N-({4-[(1S)-4-(2,4-diamino-6-oxo-1,6-dihydropyrimidin-5-yl)-1-(methylsulfanyl)butyl]phenyl}carbonyl)-L-glutamic 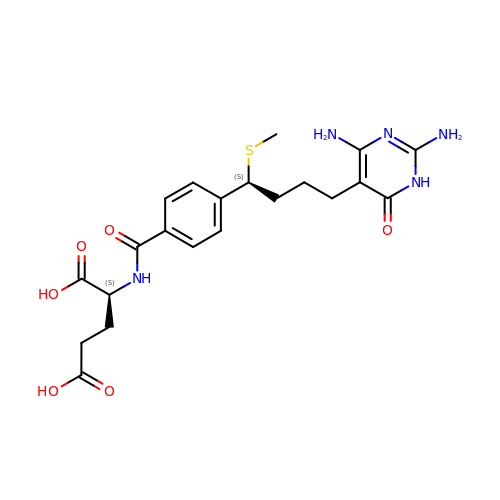acid | C21 H27 N5 O6 S | GEZLAVXTPLTVRU-GJZGRUSLSA-N>[2x]MGSSHHHHHHSSGLVPRGSSKNTGDIAIIGMAGRYPKAKSVAEFWENLKAGTDCITEVPKSRWDWKTYKNVTSPSGKTVSKWGGFIDDADCFDPQFFRISPREAETMDPQERLFLETCWETIEDAGYTPETLGNKGEKQHPIGVFAGVMHKDYSLIGAEQLSETDPFPVSLNYAQIANRVSYYCDFHGPSIAVDTVCSSSLTAVHLAIESIRRGECEAALAGG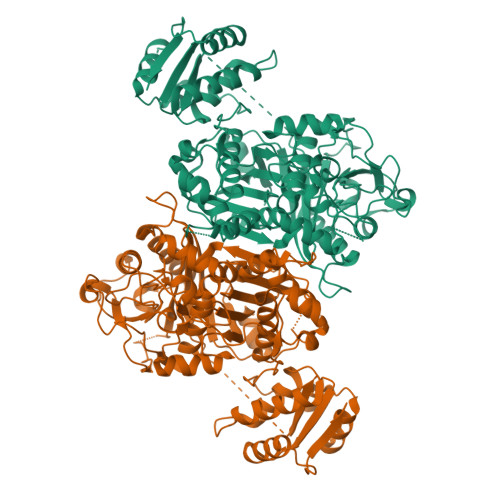VNLSLHPAKYLSYGSVGMHSSDGRCRTFGEGGDGYVSGEGVGAVLLKPLEKAEQDGDRIYAVIKGSAINHVGKVSGITVPSPAAQAEVIKACLKKAGISPRTVSYVEAHGTGTSLGDPIEIEGLSKAFSQGTQDQQFCSIGSVKSNIGHAESAAGISGLTKAALQLHHKTLVKSLHSAELNPYLKFEESPFYVQQQTAPWKQPSAEENGKVTHYPRRAGLSSFGASGSNAHIILEEYIQPEQKAPAPENEAAKLIPLSARNKDRLLAYAEKLARSLSEKTVLSELAYTIQTGREAMEERAVFLVNDIRDLKQKLNDFVKGNENIPGLWRGQAELPEMSETAPETDDSIRLAELWAEGKTVDWNKLYGSGKPRKTSVPTYPFAKERYWIPQQ> MFRRGLVHRRYPFNKRGPRERKSWKHHVLTDPPKPIQWRDPKVWTKDLTTMKSFDAPQWDLWQSRARSEDIDEALQPFMDMPQSLKDRRYDIPWWANPFGAWYLQNILSVELLKLPSRTNAEKVAIYRNQKHSLSSKKKGEAAQDDEILANIIKERWRTLEFGDRDAGYPCTFSDYIQFLNEWFKSLDEEGMQRLREHFDRRIRPLLAVMSPVDILWLEALTQNSPHNKEQLQRRIAFQTSLGTPEFFDMSKRLRYEINEDYKVRDELGPELFALWSKAPERWPPERLSKMYGLDFTLVRKILVWHHFKACYDACVEPDWTLPKRLFALEWIRDVRARKHGLFYGKMRFAEQKITFYSDRFLFRDLVNRREASYANVWEMDDPYRFLQTEQDYEDYWGDNYDVYRRMFPEMIGKSGEPVQQYGQMPVWTGPHRQHANKSQHNWMFAEIGVNVGHEALKKLELDPTNEKRRRFVIRQPDGTLRSAKMSEMRAWYWKEEWADFRFWAPNMEWGIENT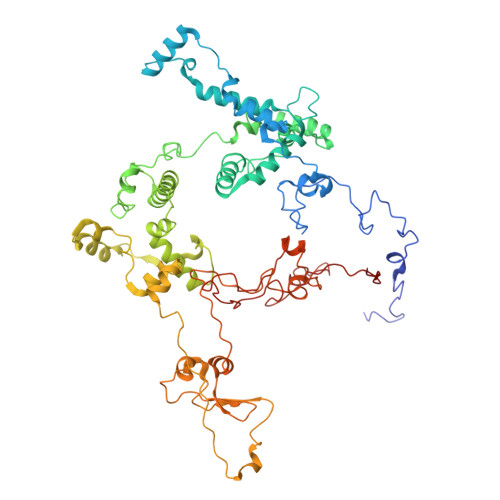PSQEQYQEHVPDTPDADFRKQRRIQSRPVKWFYESHYTRTGNFAGFQPLRFMQRRTEREVRWPDVINAAVQIQKRKPDAYIFKAIPEI>MPFVKDFKPQALGDTNLFKPIKIGNNELLHRAVIPPLTRMRAQHPGNIPNRDWAVEYYAQRAQRPGTLIITEGTFPSPQSGGYDNAPGIWSEEQIKEWTKIFKAIHENKSFAWVQLWVLGWAAFPDTLARDGLRYDSASDNVYMNAEQEEKAKKANNPQHSITKDEIKQYVKEYVQAAKNSIAAGADGVEIHSANGYLLNQFLDPHSNNRTDEYGGSIENRARFTLEVVDAVVDAIGPEKVGLRLSPYGVFNSMSGGAETGIVAQYAYVLGELERRAKAGKRLAFVHLVEPRVTNPFLTEGEGEYNGGSNKFAYSIWKGPIIRAGNFALHPEVVREEVKDPRTLIGYGRFFISNPDLVDRLEKGLPLNKYDRDTFYKMSAEGYIDYPTYEEALKLGWDKN[2x]

A family of flavin-containing ene-reductases (EREDs) named old yellow enzymes (OYEs) have been studied for close to a century, yet continue to surprise with its versatile activities. Typically, OYEs reduce activated alkenes asymmetrically following a bi-bi ping-pong mechanism, in which a reduced nicotinamide cofactor reduces the flavin followed by a flavin hydride attack on the substrate’s β-carbon with a local tyrosine as a proton donor. OYEs are classified into several classes: class I are from plants, cyano-, actino-, and proteobacteria, class II are the classical OYEs from fungi, and class III are similar to class I species but are thermophilic-like OYEs, and so far classes IV–VI are less defined. EREDs are able to catalyze the asymmetric monoreduction of α,β-dicarbonyl compounds toward α-hydroxy carbonyls.

A second study showed OYEs mediate vicinal dicarbonyl reduction;9 however, the focus was narrowed to two enzymes from class II, OYE2 and OYE3 from Saccharomyces cerevisiae showing kinetic data only, without knowledge of the enzymatic product and enantioselectivity. Despite numerous attempts at cocrystallization or crystal soaking of OYE2 and OYE3 with 7a, no interpretable electron density was observed in the active site corresponding to the substrate. A new structure of OYE2 was solved at a resolution of 1.5 Å resolution, higher than the previously published 2.45 Å,40 and molecular docking was performed with 7a. Semiflexible dockings were performed whereby 7a was allowed to sample various conformations, with the condition that only the side chains of amino acids lining the active site of the OYEs were allowed to move (semi-induced fit). Productive binding conformations were considered if one of the carbonyl groups was hydrogen bonded to the active site Asn-His pair. 7a was docked into OYE2 with the β-carbonyl hydrogen bonded to the Asn-His pair, and the carbonyls in a cis configuration. The benzene ring of 7a is in an edge-to-face position relative to both FMN and F297. The dihedral angle between the two carbonyl groups in OYE2 is only ca. 18°, which would suggest a high energy conformation for 7a. This could, however, be mediated by the hydrogen bonding of the β-carbonyl group to the Asn-His pair. Alternatively, if 7a were to adopt a lower potential energy by rotation of the intercarbonyl bond, this would place the α-carbonyl oxygen closer to the N5 of FMN.>MVVIDLLIVEVVLFIAALLFSGFFSSSEVALISITRAKVHALQSQGRKGAKALDTLKRSTDAIQITTLIGSTIANVAVASLATAIGITLYGNLGIAVGLVVAAVLVLVFGEIGPKMYASRYTEELALRVSRPILFFSKLLYPVLWVTDRIEQQFAFRPGVTEPVVTEEEIKEWIDVGEEEGTIEEEERDMLYSVLRFGDTTAREVMTPRVDVVMIEDTATLESALAIFNETGFSLIPVYHERIDNIVGLLNVKDVFSAVFRQQTSATIRDLMYEPYFIPESKKIDELLKELQVKKQH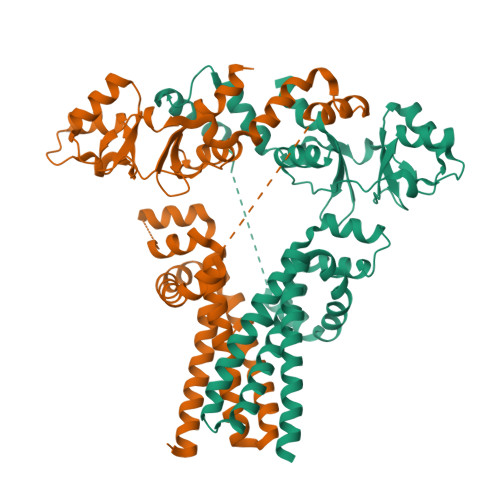MAVVLDEYGSFAGIVTVEDMLEELVHHHHHH[2x]> GSHMEVLKNIRIYPLSNFITSTKNYINLPNELRNLISEEQESKLGFLHIIESDFKPSVALQKLVNCTTGDEKILIIDIVSIWSQQKQRQHGAIYMNSLSCINITGLIVFLELLYDSPMDALRRCQVDNFNFQLRGIVIDNLSFLNFESDKNYDVINLSKFE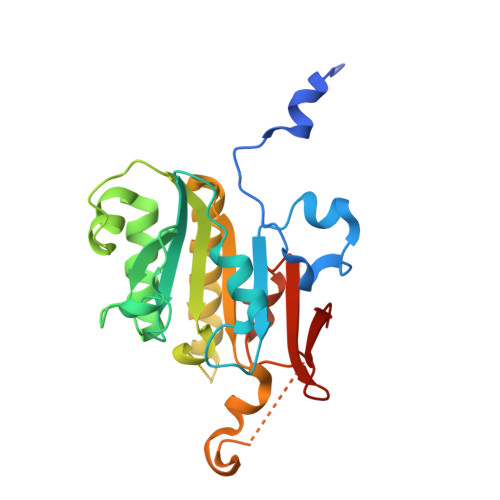KLFKILRKLREFLGCWIITKSFPTDFYNGIENTLVDKWSIKRKSGVTLYPTKLPDSYMKGMDLIIYREVVDGRPQYRRIAALEE> MRPYTLSVALPGSILDNAQSPELRTYLAGQIARACAIFCVDEIVVFDEEGQDAKTVEGEFTGVGKKGQACVQLARILQYLECPQYLRKAFFPKHQDLQFAGLLNPLDSPHHMRQDEESEFREGIVVDRPTRPGHGSFVNCGMKKEVKIDKNLEPGLRVTVRLNQQQHPDCKTYHGKVVSSQDPRTKAGLYWGYTVRLASCLSAVFAEAPFQDGYDLTIGTSERGSDVASAQLPN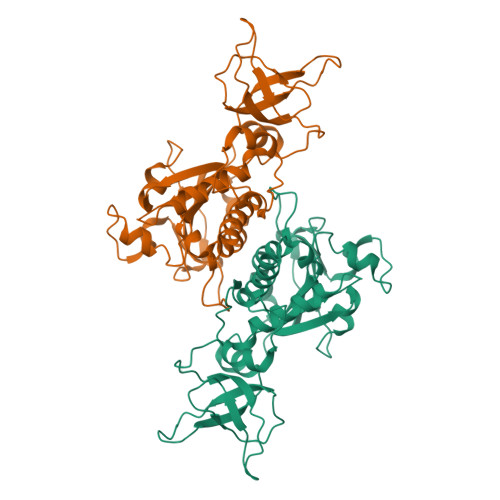FRHALVVFGGLQGLEAGADADPNLEVAEPSVLFDLYVNTCPGQGSRTIRTEENILISLAALQPGLIQAGARHT> SVENHWYYF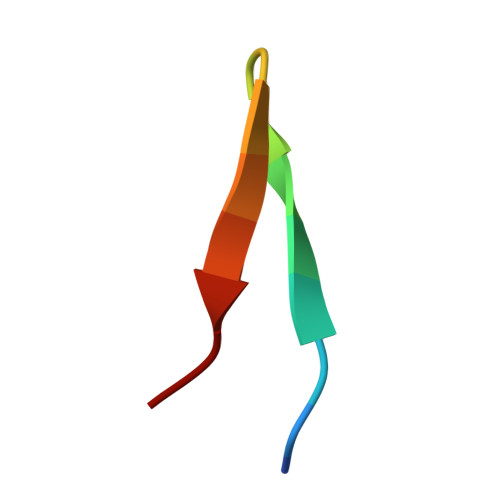YWYMSP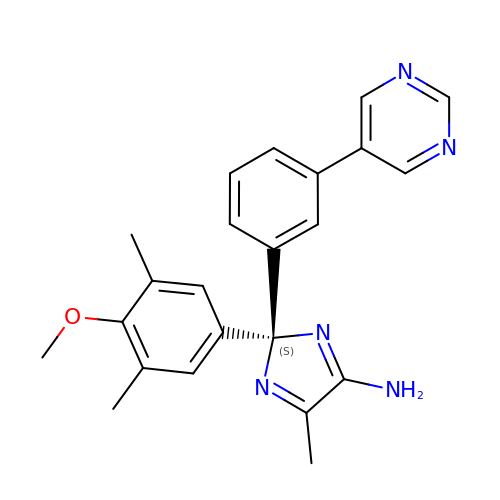(2S)-2-(4-methoxy-3,5-dimethylphenyl)-5-methyl-2-(3-pyrimidin-5-ylphenyl)-2H-imidazol-4-amine | C23 H23 N5 O | PZSMDBYYYKPYFV-QHCPKHFHSA-N The ω-transaminase from Vibrio fluvialis JS17 (Vfat) is an unique PLP-containing enzyme that catalyzes the reversible amino group transfer reaction from an amine to a keto acid. Vfat is an amine:pyruvate transaminase capable of the stereo-selective transamination of arylic chiral amines that is highly suitable for the production of chiral amines due to its strict enantio-selectivity and its broad specificity for chiral amine amino donors. All transaminases use pyridoxal 5ʹ-phosphate (PLP) as a cofactor for catalysis. The overall structure of apo Vfat shows the typical transaminase fold, which is comprised of two major domains, the small domain and the large domain.

In the present study, we report the crystal structure of the PLP free apo Vfat. Two molecules, subunit A and subunit B, were detected in the asymmetric unit. Interestingly, the two subunits did not contain any cofactor such as PMP or PLP based on the electron density map. As the dimeric form of the current structure might be coincidently formed during crystal packing, we confirmed the stoichiometry of the apo-state of Vfat in solution by multi-angle light scattering (MALS), which measures the absolute molecular mass of the target protein in solution. The theoretical molecular mass of Vfat, including the His-tag was 52.79 kDa, whereas the measured mass was 103.72 kDa (0.89% fitting error), indicating that the apo-state of Vfat also forms a dimer in solution. The structure of the two PLP/PMP bound Vfats differed from our apo Vfat structure in that both of the two cofactor-bound forms (PLP/PMP) of Vfat had structurally stable helices in the α1-α2 region and the α6-α7 region unlike the cofactor free Vfat form whose structure contained a disordered α1-α2 region in subunit A and a disordered α6-α7 in subunit B. The PLP/PMP bound Vfat had four symmetric molecules in the asymmetric unit. Interestingly, however, the two subunits in the apo form of Vfat showed different side chain orientation at K285 despite the backbone folding in the vicinity of the K285 in both subunits being structurally analogous to those of the PLP- and PMP-bound form. Specifically, the side chain group of K285 in subunit A showed a similar orientation to that of PMP-bound form, whereas the side chain group of K285 in subunit B had the opposite orientation. After careful analysis of the structure, and by lowering the contours of the Fo-Fc map, we discovered a small volume of electron density around the substrate pocket of subunit A. After several rounds of restrained refinement with Refmac5, we determined the electron density for the small molecule to be around the substrate pocket in subunit A. In addition, a small molecule in the apo state of Cv-ωTA was not found in the substrate pocket.

>MASMTGGQQMGRGSMNKPQSWEARAETYSLYGFTDMPSLHQRGTVVVTHGEGPYIVDVNGRRYLDANSGLWNMVAGFDHKGLIDAAKAQYERFPGYHAFFGRMSDQTVMLSEKLVEVSPFDSGRVFYTNSGSEANDTMVKMLWFLHAAEGKPQKRKILTRWNAYHGVTAVSASMTGKPYNSVFGLPLPGFVHLTCPHYWRYGEEGETEEQFVARLARELEETIQREGADTIAGFFAEPVMGAGGVIPPAKGYFQAILPILRKYDIPVISDEVICGFGRTGNTWGCVTYDFTPDAIISSKNLTAGFFPMGAVILGPELSKRLETAIEAIEEFPHGFTASGHPVGCAIALKAIDVVMNEGLAENVRRLAPRFEERLKHIAERPNIGEYRGIGFMWALEAVKDKASKTPFDGNLSVSERIANTCTDLGLICRPLGQSVVLCPPFILTEAQMDEMFDKLEKALDKVFAEVAAA[2x]>[2x]GMIISLIAALTENRVIGKSNDLPWHLPDDMKYFMQTTLGHHVIMGRKNYESIPAKFRPLANRTNIVVTRQEEYDAAGCIVVNSIPAGIDIAIDNREAEVFIIGGAEIYTQSLAFA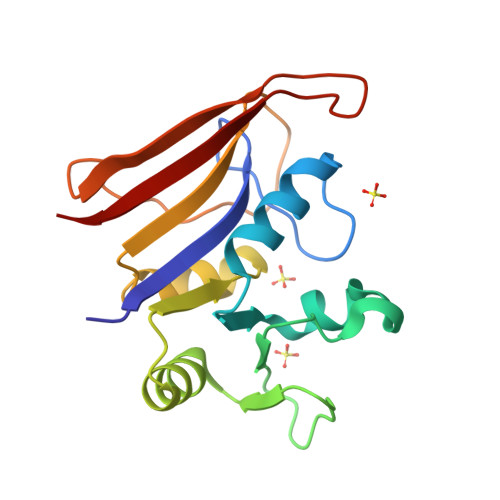NRLYLTEIQTSLEGDAFFPMFNKHEWNELSRKHHPLDEKHRYSFDFVIYEKK>[2x]GPDEIDLSALRDPAGIFELVELVGNGTYGQVYKGRHV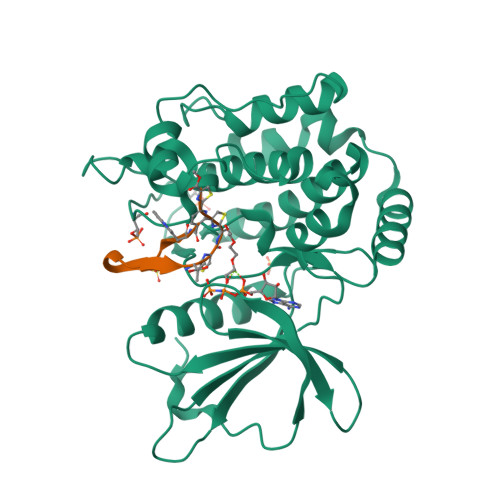KTGQLAAIKVMDVTGDEEEEIKQEINMLKKYSHHRNIATYYGAFIKKNPPGMDDQLWLVMEFCGAGSVTDLIKNTKGNTLKEEWIAYICREILRGLSHLHQHKVIHRDIKGQNVLLTENAEVKLVDFGVSAQLDRTVGRRNTFIGTPYWMAPEVIACDENPDATYDFKSDLWSLGITAIEMAEGAPPLCDMHPMRALFLIPRNPAPRLKSKKWSKKFQSFIESCLVKNHSQRPATEQLMKHPFIRDQPNERQVRIQLKDHIDRTKKKRG;>SWTIRTRGRIATCSCSCX[2x]>MVDLKRLRQEPEVFHRAIREKGVALDLEALLALDREVQELKKRLQEVQTERNQVAKRVPKAPPEEKEALIARGKALGEEAKRLEEALREKEARLEALLLQVPLPPWPGAPVGGEEANREIKRVGGPPEFSFPPLDHVALMEKNGWWEPRISQVSGSRSYALKGDLALYELALLRFAMDFMARRGFLPMTLPSYAREKAFLGTGHFPAYRDQVWAIAETDLYLTGTAEVVLNALHSGEILPYEALPLRYAGYAPAFRSEAGSFGKDVRGLMRVHQFHKVEQYVLTEASLEASDRAFQELLENAEEILRLLELPYRLVEVATGDMGPGKWRQVDIEVYLPSEGRYRETHSCSALLDWQARRANLRYRDPEGRVRYAYTLNNTALATPRILAMLLENHQLQDGRVRVPQALIPYMGKEV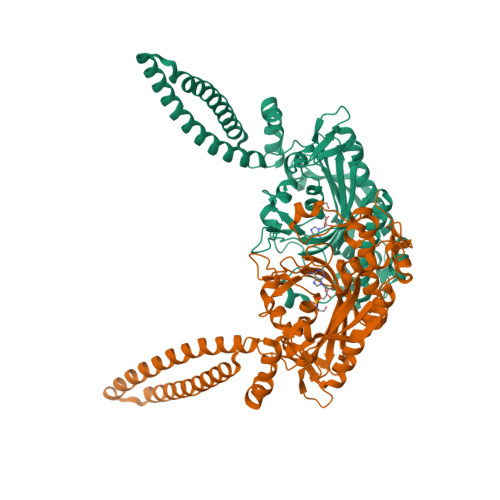LEPCG[2x]>EGDIHMKKGHHHHHHENLYFQGGSGKLSEQLKHCNGILKELLSKKHAAYAWPFYKPVDASALGLHDYHDIIKHPMDLSTVKRKMENRDYRDAQEFAADVRLMFSNCYKYNPPDHDVVAMARKLQDVFEFRYAKMP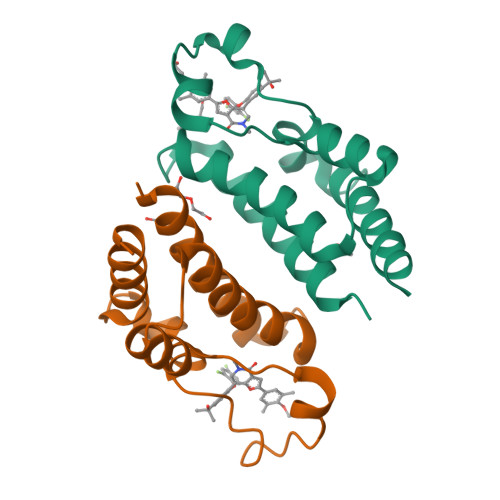D[2x]>MPHDVHIEMTAQITDIEIDKGKIYKAWTFNGQAPGPLVVVNEGDTIHFTLKNMDPVVPHSMDFH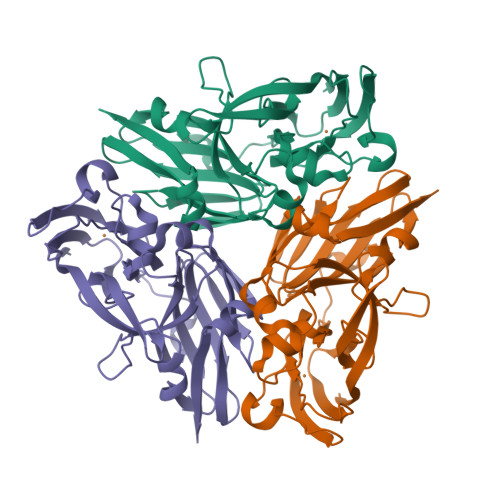AVHASPSKDFIDVMPNKSGTFTYPANKPGVFMYHCGTKPVLQHIANGMHGVIIVKPKNGYPTDKEVDREYVLIQNEWYKYNDMNDFQNGVPSYVVFSSKALKPGDPNTNGDTFTLKEKPLLAKVGEKIRLYINNVGPNEVSSFHVVGTVFDDVYLDGNPNNHLQGMQTVMLPASGGAVVEFTVTRPGTYPIVTHQFNHAQKGAVAMLKVTETGEDDGSETSGH[9x]>MSQSGEDLHSPTYLSWRKLQLSRAKLKASSWTSALLSGFAMVAMVEVQLDHDTNVPPGMLIAFAICTTLLVAVHMLALMISTCILPNIETVSNLHSISLVHESPHERLHWYIETAWAFSTLLGLILFLLEIAILCWVKFYDLSPPAAWSATVVLIPVMIIFMAFAIHFYRSLVSHKYEVTVSGIRELEMLKEQMEQDHLEHHN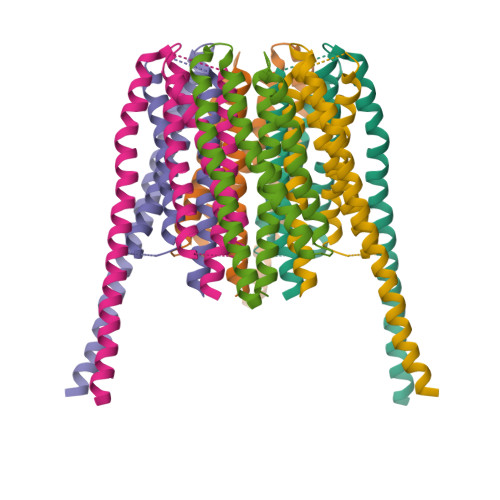NIRNNGEGEEF[3x]> UCCCAGUCCAC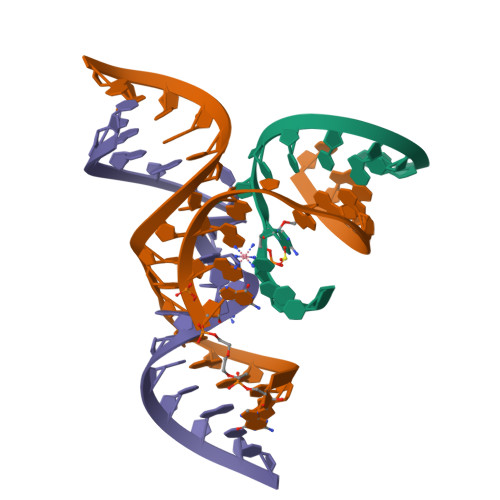CGU;> CGGUGAGXAGGGXGGCAGAGAAACACACGA;> UCGUGGUACAUUACCUGCC> MHHHHHHLPNITILATGGDIAGGGDSATKSNYTVGKVGVENLVNAVPQLKDIANVKGEQVVNIGSQDMNDNVWLTLAKKINTDCDKTDGFVITHGTDTMEETAYFLDLTVKCDKPVVMVGAMRPSTSMSADGPFNLYNAVVTAADKASANRGVLVVMNDTVLDGRDVTMTNTTDVATFKSVNYGPLGYIHNGKIDYQRTPARKHTSDTPFDVSKLNELPKVGIVYNYANASDLPAKALVDAGYDGIVSAGVGNGNLYKSVFDTLATAAKTGTAVVRSSRVPTGATTQDAEVDDAKYGFVASGTLNPQKARVLLQL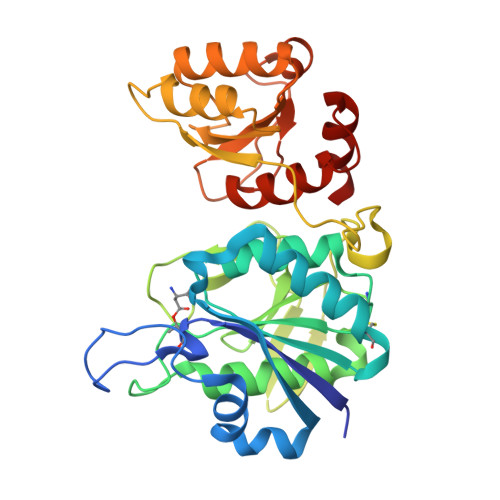ALTQTKDPQQIQQIFNQY>XGELKAIAQELKAIAKECKAIAYELKAIAQGAG[3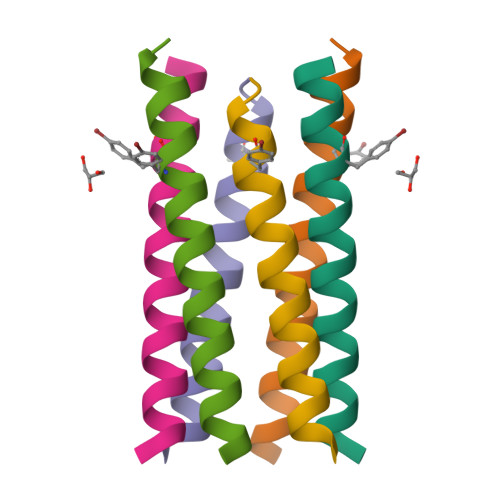x]EttA, energy-dependent translational throttle A, is a ribosomal factor that gates ribosome entry into the translation elongation cycle. Here we present the cryo-electron microscopy (cryo-EM) structures of EttA from Mycobacterium tuberculosis (Mtb), referred to as MtbEttA, in complex with the Mtb 70S ribosome initiation complex (70SIC) at the pre-hydrolysis (ADPNP) and transition (ADP-VO4) states, and the crystal structure of MtbEttA alone in the post-hydrolysis (ADP) state. We observe that MtbEttA binds the E-site of the Mtb 70SIC, remodeling the P-site tRNA and the ribosomal intersubunit bridge B7a during the ribosomal ratcheting. MtbEttA has a conserved ABC-F architecture with two tandem NBDs, an arm domain, PtIM, and a basic C-terminal tail.

Based on our result, MtbEttA in the ADP state did not form a stable complex with the ribosome. Therefore, we co-crystalized MtbEttA with ADP and determined its X-ray crystal structure at 2.9 Å resolution. In the crystal, the asymmetric unit of MtbEttA-ADP consists of a domain-swapped dimer, similar to that in the crystal structure of nucleotide-free EcoEttA. In the crystal structure of the post-hydrolysis state of MtbEttA, one ADP molecule and a Mg2+ ion are clearly resolved in each of the four NBSs in the domain-swapped dimer. To measure the conformational difference, we align the two structures of MtbEttA in the post-hydrolysis (ADP) state and the Trans_R0 state based on the NBD1. We observe a ~40o rotation of NBD2 away from NBD1 in the post-hydrolysis state, allowing the formation of two new salt bridges (E199/R499 and R216/E482) between NBD1 and NBD2. In order to evaluate the effects of such a large domain movement of MtbEttA at the post-hydrolysis state, we superimposed the structure of the two NBDs of MtbEttA in the ADP state to the 70SIC-MtbEttA complex in the Trans_R0 state based on NBD1. Clear steric clashes are observed between the NBD2 and arm domain with uS7 and uL1, respectively. This may explain why the ADP-state MtbEttA cannot form a stable complex with the Mtb 70SIC and has to dissociate from the ribosome after ATP hydrolysis.

>[2x]MAEFIYTMKKVRKAHGDKVILDDVTLSFYPGAKIGVVGPNGAGKSSVLRIMAGLDKPNNGDAFLATGATVGILQQEPPLNEDKTVRGNVEEGMGDIKIKLDRFNEVAELMATDYTDELMEEMGRLQEELDHADAWDLDAQLEQAMDALRCPPADEPVTNLSGGERRRVALCKLLLSKPDLLLLDEPTNHLDAESVQWLEQHLASYPGAILAVTHDRYFLDNVAEWILELDRGRAYPYEGNYSTYLEKKAERLAVQGRKDAKLQKRLTEELAWVRSGAKARQAKSKARLQRYEEMAAEAEKTRKLDFEEIQIPVGPRLGNVVVEVDHLDKGYDGRALIKDLSFSLPRNGIVGVIGPNGVGKTTLFKTIVGLETPDSGSVKVGETVKLSYVDQARAGIDPRKTVWEVVSDGLDYIQVGQTEVPSRAYVSAFGFKGPDQQKPAGVLSGGERNRLNLALTLKQGGNLILLDEPTNDLDVETLGSLENALLNFPGCAVVISHDRWFLDRTCTHILAWEGDDDNEAKWFWFEGNFGAYEENKVERLGVDAARPHRVTHRKLTRG>[3x]MAKRLSKQQLAKAIANTLETPPQPKAGRRRNRRRQRSAVQQLQPTQAVRIRNPAVSSSRGGITVLTHSELSAEIGVTDSIVVSSELVMPYTVGTWLRGVAANWSKYSWLSVRYTYIPSCPSSTAGSIHMGFQYDMADTVPVSVNQLSNLRGYVSGQVWSGSAGLCFINGTRCSDTSTAIS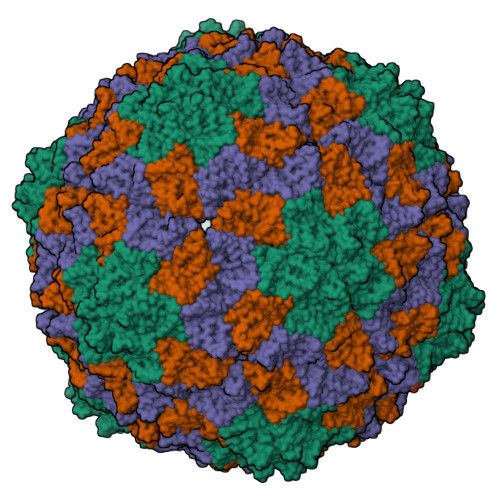TTLDVSKLGKKWYPYKTSADYATAVGVDVNIATPLVPARLVIALLDGSSSTAVAAGRIYCTYTIQMIEPTASALNN> MSAALPSIQLPVDYNNLFNEITDFLVTFKQDTLSSDATRNENEDENLDAENIEQHLLEKGPKYMAMLQKVANRELNSVIIDLDDILQYQNEKFLQGTQADDLVSAIQQNANHFTELFCRAIDNNMPLPTKEIDYKDDVLDVILNQRRLRNERMLSDRTNEIRSENLMDTTMDPPSSMNDALREVVEDETELFPPNLTRRYFLYFKPLSQNCARRYRKKAISSKPLSVRQIKGDFLGQLITVRGIITRVSDVKPAVEVIAYTCDQCGYEVFQEVNSRTFTPLSECTSEECSQNQTKGQLFMSTRASKFSAFQECKIQELSQQVPVGHIPRSLNIHVNGTLVRSLSPGDIVDVTGIFLPAPYTGFKALKAGLLTETYLEAQFVRQHKKKFASFSLTSDVEERVMELITSGDVYNRLAKSIAPEIYGNLDVKKALLLLLVGGVDKRVGDGMKIRGDINVCLMGDPGVAKSQLLKAICKISPRGVYTTGKGSSGVGLTAAVMKDPVTDEMILEGGALVLADNGICCIDEFDKMDESDRTAIHEVMEQQTISISK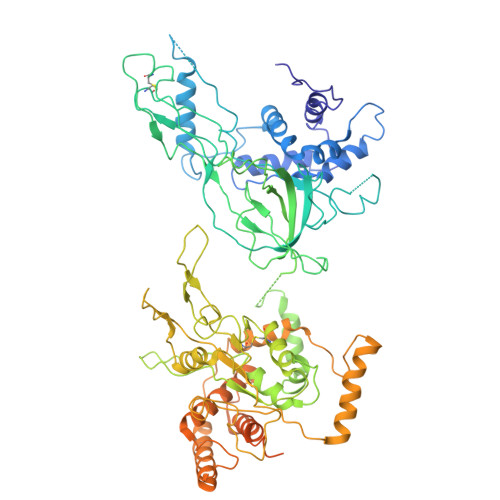AGINTTLNARTSILAAANPLYGRYNPRLSPLDNINLPAALLSRFDILFLMLDIPSRDDDEKLAEHVTYVHMHNKQPDLDFTPVEPSKMREYIAYAKTKRPVMSEAVNDYVVQAYIRLRQDSKREMDSKFSFGQATPRTLLGIIRLSQALAKLRLADMVDIDDVEEALRLVRVSKESLYQETNKSKEDESPTTKIFTIIKKMLQETGKNTLSYENIVKTVRLRGFTMLQLSNCIQEYSYLNVWHLINEGNTLKFVDDGTMDTDQEDSLVSTPKLAPQTTASANVSAQDSDIDLQDA>MITLTTDFGLKGPYVGEMKVAMLRINPNAKIVDVTHSVTRHSILEGSFVMEQVVKYSPKGTVHVGVIDPGVGTERRAIVIEGDQYLVVPDNGLATLPLKHIKVKSVYEIIPDKIRKFTGWEISSTFHGRDIFGPAGALIEKGIHPEEFGREIPVDSIVKLNVEPRKEGDVWILKVIYIDDFGNVILNLENYEKPRTVELLDFNLRLPYLETYGLVEKGEMLALP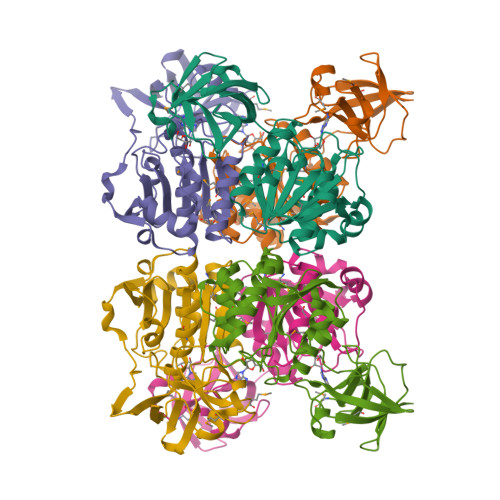GSHDYLEIAVNMGSAAERLNVKVGDELRVRLL[3x]Previously, we utilized this platform to identify a series of thiopeptides acting as potent and selective inhibitors of Traf2- and NCK-interacting kinase (TNIK), a protein implicated in several forms of cancer. However, the discovered thiopeptides featured random inserts composed predominantly of proteinogenic amino acids, which limited their likeness to natural products and led to modest metabolic stabilities. We demonstrate the feasibility of our designs by conducting affinity selections against Traf2- and NCK-interacting kinase (TNIK). An X-ray cocrystal structure of TNIK in complex with a discovered thiopeptide revealed how nonproteinogenic building blocks facilitate the target engagement and orchestrate the folding of the thiopeptide into a noncanonical conformation. X-ray structural analysis of the interaction between TNIK and one of the discovered thiopeptides, wTP3, pointed to a predominantly hydrophobic association driven by the steric complementarity between the protein and ligand.

To understand how densely functionalized thiopeptides interact with their target proteins, we solved the X-ray crystal structure of the TNIK·AMPPNP·wTP3 complex at 2.8 Å resolution. Like the previously identified TP1 and TP15 thiopeptides, wTP3 binds to the substrate binding site of TNIK. However, the binding mode of wTP3 deviates from those of TP1 and TP15.33 The peptide contacts both the N- and C-lobes of TNIK, interacting primarily with the αG-helix and P+1 loop in the C-terminal lobe. The N-lobe amino acids, Asp61-Glu62 in the αC-helix and Thr35-Tyr36 in the Gly-rich loop, additionally contact TicOH8-Dha9 residues in wTP3. The hydrogen bond between the side chain carboxylate of Glu62 and the amide nitrogen of Dha9 is the only polar contact in the interface, and the near absence of polar interactions between the protein and wTP3 is a striking feature of the structure. Instead, the high steric complementarity of wTP3 and TNIK appears to drive the association. Trp2, Trp3, and N-Me-Gly5 of wTP3 make numerous contacts with the exposed hydrophobic patch on the surface of TNIK. The carbonyl oxygen of Trp3 and the N-Me group of N-Me-Gly5 occupy the P+1 site, whereas the indole groups of Trp2 and Trp3 are stacked against the αG-helix residues, primarily His237, Pro238, Met239, and Leu242. Another notable feature of the structure is the intramolecular interactions and folding of wTP3. The pyridine-diazole moiety, the side chains of N-Me-Nph12, and Thr11 as well the phenol in TicOH8 are stacked on top of each other providing π–π and CH-π interactions which appear to rigidify and stabilize the peptide structure. wTP3 folds into a unique “quadruply twisted” conformation featuring two β-turns and two noncanonical turn elements organized without the use of intramolecular hydrogen bonds owing to the multiple nonproteinogenic elements in the structure.

> GPDEIDLSALRDPAGIFELVELVGNGTYGQVYKGRHVKTGQLAAIKVMDVTGDEEEEIKQEINMLKKYSHHRNIATYYGAFIKKNPPGMDDQLWLVMEFCGAGSVTDLIKNTKGNTLKEEWIAYICREILRGLSHLHQHKVIHRDIKGQNVLLTENAEVKLVDFGVSAQLDRTVGRRNTFIGTPYWMAPEVIACDENPDATYDFKSDLWSLGITAIEMAEGAPPLCDMHPMRALFLIPRNPAPRLKSKKWSKKFQSFIESCLVKNHSQRPATEQLMKHPFIRDQPNERQVRIQLKDHIDRTKKKRG At the molecular level, the mammalian circadian clock operates through an auto-regulatory transcription–translation feedback loop composed of four core components—the transcriptional activator proteins, CLOCK and BMAL1, and the transcriptional repressors, Periods (PERs) and Cryptochromes (CRYs). The PER and CRY proteins function as the negative arm of the loop by blocking the activity of CLOCK-BMAL1 and inhibiting the transcription of their own and all other clock-controlled genes. Mammalian PER1 and PER2 share ∼50% sequence identity and a common domain architecture comprised of tandem N-terminal PER-ARNT-SIM (PAS) domains, a central CK1δ/ε-binding region, and a ∼100 amino acid long C-terminal CRY-binding domain (CBD), which is necessary and sufficient for CRY binding. Here, we report the crystal structure of a PER2–CRY2 complex, which provides the missing structural framework for understanding the multiple functions of PERs in driving the molecular clock.

PER2-CBD adopts a highly extended structure, devoid of a hydrophobic core. In the crystal, PER2-CBD meanders along one side of CRY2-PHR and sinuously wraps around the region. With nearly half of the PER2 residues involved in binding, the two proteins bury a total 2800 Å2 of solvent accessible surface area at the interface, which stretches over a distance of more than 215 Å. In comparison to its FBXL3-, KL001-, and FAD-complexed forms, CRY2 adopts the same global fold when bound to PER2-CBD. The largest structural variations take place in two local regions, the interface loop next to the FAD-binding pocket and a serine-rich loop neighboring a secondary pocket (see below). The PER2-CBD α3 helix preceding this loop packs against the long CRY2 C-terminal helix at an approximately 30° angle, while the region C-terminal to the loop locks onto the same CRY2 helix from the other side. Together, these PER2-CBD structural elements encircle the CRY2 C-terminal helix like an U-shaped clamp. Superposition analysis reveals that FBXL3 and PER2 cannot be simultaneously engaged with CRY2 without clashing into each other. In the complex structure, these two cysteine (C1210 and C1213) residues face a pair of cysteine and histidine residues in CRY2 (C432 and H491), which are also invariant among vertebrate CRY1/2 proteins. Together, these four residues sequester a strong density at the center, hinting at the coordination of a Zn2+ ion at the end of the PER2–CRY2 interface.

>[2x]MAAAAVVAATVPAQSMGADGASSVHWFRKGLRLHDNPALLAAVRGARCVRCVYILDPWFAASSSVGINRWRFLLQSLEDLDTSLRKLNSRLFVVRGQPADVFPRLFKEWGVTRLTFEYDSEPFGKERDAAIMKMAKEAGVEVVTENSHTLYDLDRIIELNGQKPPLTYKRFQALISRMELPKKPAVAVSSQQMESCRAEIQENHDDTYGVPSLEELGFPTEGLGPAVWQGGETEALARLDKHLERKAWVANYERPRMNANSLLASPTGLSPYLRFGCLSCRLFYYRLWDLYKKVKRNSTPPLSLFGQLLWREFFYTAATNNPRFDRMEGNPICIQIPWDRNPEALAKWAEGKTGFPWIDAIMTQLRQEGWIHHLARHAVACFLTRGDLWVSWESGVRVFDELLLDADFSVNAGSWMWLSCSAFFQQFFHCYCPVGFGRRTDPSGDYIRRYLPKLKGFPSRYIYEPWNAPESVQKAAKCIIGVDYPRPIVNHAETSRLNIERMKQIYQQLS;>SSDTSHTSKYFGSIDSSENNHKAKMIPDTEESEQFIKYVLQDPIWLLMANTDDSIMMTYQLPSRDLQAVLKEDQEKLKLLQRSQPRFTEGQRRELREVHPWVHTGGLPTAIDVTGCVYCES[2x]>[9x]SDFVVIKALEDGVNVIGLTRGADTRFHHSEKLDKGEVLIAQFTEHTSAIKVRGKAYIQTRHGVIE

Here we examined the factors that define the oligomeric state in a circular protein oligomer by studying the Bacillus trp RNA-binding attenuation protein (TRAP). Studies on B. subtilis have shown that when TRAP is activated by bound tryptophan, it can recognize and bind specific segments of RNA. When the tryptophan concentration is high transcription attenuation occurs as TRAP, binding to the leader RNA region of the trpEDCFBA operon transcript, induces the formation of a transcription terminator hairpin thus preventing the establishment of an antiterminator structure. When the concentration of tryptophan is limiting, TRAP is inactive, which allows transcription to proceed into the structural genes.

We hypothesized that the 11-mer to 12-mer switch could be induced by withdrawal of the C-terminal amino acids from the subunit-subunit interface, as observed in B. halodurans TRAP. Such a switch could be engineered by simply removing the C-terminal amino acids starting from position 72. We tested this idea using B. stearothermophilus TRAP which normally forms 11-mers. The E71stop B. stearothermophilus TRAP mutant protein was truncated after residue 71 thus removing the five C-terminal amino acids and the main chain hydrogen bond between Gly41 and Glu73. The conformation of individual subunits is also very similar, with the main chain r.m.s. difference with the B. halodrurans TRAP (residues 8–65) of 0.38 Å and 0.33 Å, respectively, for the engineered B. stearothermophilus and B. subtilis TRAP. The engineered 12-mer TRAP share almost identical intersubunit hydrogen bonding patterns with those in wild type 11-mers, Tables S2 and S3. We questioned whether the 12-subunit assemblies of B. halodurans TRAP and B. stearothermophilus E71stop TRAP predominate in solution or whether these were selected from a mixture of different oligomeric states during crystallization.>MGNAKTRRRERRAEKQAQWKAANAGAGAGAMATPHFDYIASEVSKGLANLSLELRKPITFGVITADTLEQAIERAGTKHGNKGWEAALSAIEMANLFKSLRGTGHHHHHHGSSMEIYEGKLTAEGLRFGIVASRFNHALVDRLVEGAIDCIV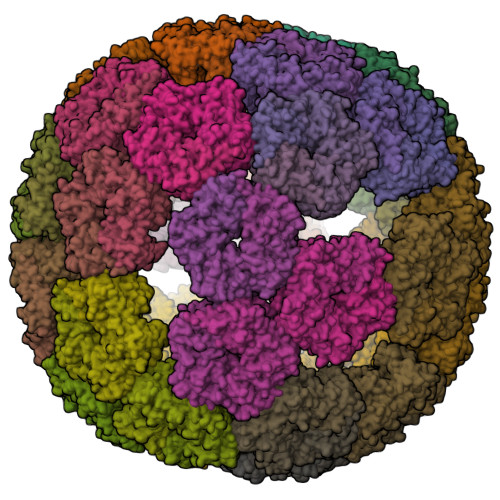RHGGREEDITLVRVPGSWEIPVAAGELARKEDIDAVIAIGVLIRG[180x]> GSMTEADVNPKAYPLADAHLTKKLLDLVQQSCNYKQLRKGANEATKTLNRGISEFIVMAADAEPLEIILHLPLLCE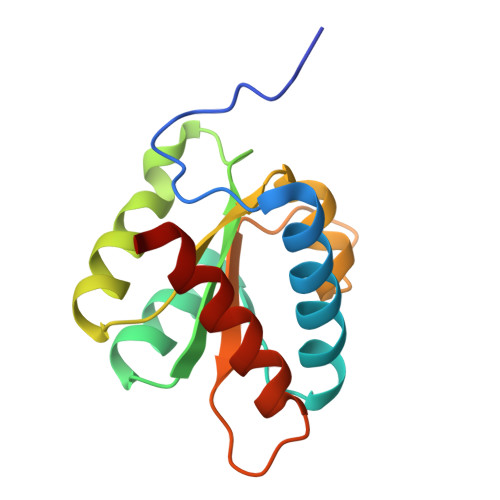DKNVPYVFVRSKQALGRACGVSRPVIACSVTIKEGSQLKQQIQSIQQSIERLLV>MADKELKFLVVDDFSTMRRIVRNLLKELGFNNVEEAEDGVDA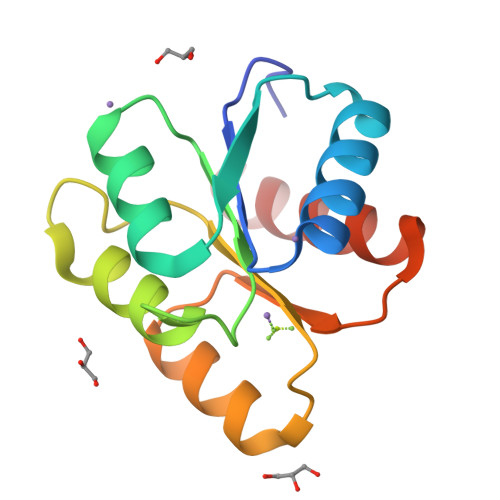LNKLQAGGYGFVISDWNMPNMDGLELLKTIRADGAMSALPVLMVTMEAKKENIIAAAQAGASGYVVKPFTAATLEEKLNKIFEKLGM[2x]>[2x]MGSSHHHHHHSSGLVPRGSMTSSPATASPAVADQLDSLAALLTSRA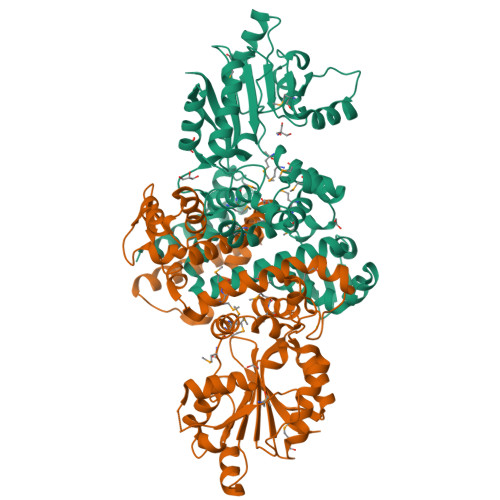QAVRNGAAVPPQQHVQLVKGLKDAAGLVNEAREDLGDLMMSFVQVTALRLLIKWKVFEAIPLEGTISYADVAARVGIDVNLITRLSWVLVATGVLKQDGSDKIQHTARSRPYASRNPLSAMMIIGFDEYLPALLAMPGYFDTYGKKEPFGEKHTVKAFSEGNPELTVNQILASSPERLGNMTLAMAAMENMYPLSGVYDFSWVAAKAASDSNRPLIVDVGGAKGHTLQAICKDTPALPIERCVLEDLPRVIQVVKDTSDAGAQAPQLLGMDFNQEQPVKGAVVYLIRRCLHDYSDEQCVRILGHLAAAMAADSVLLIGETVLTNPPSRPTAMMDILLATIGGKERTIDAFGAVVGRAGLRIKGVCKQEGGDFSYIECVKA> HHHHHHTPSTSVIPNDAIRLNQLGYYPNQEKIAVVDSGKVEEFVIWDAVSGEQVFVGKSLYTAKSAWSDKTRTTLDFSAVTTPGKYILKVNGASVTFLIKDSVLSPLA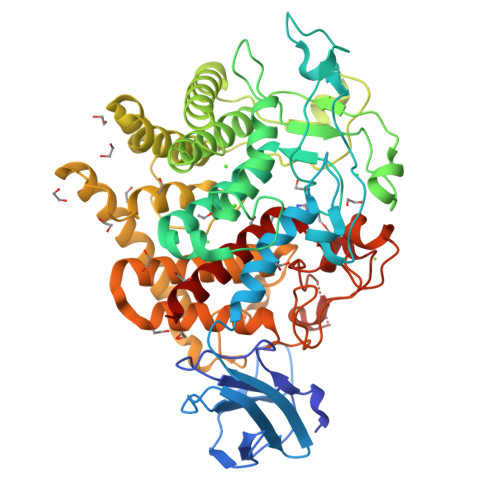DAALKSFYYQRTAMPIEEQYAGQWHRMAGHPDNHVLIHPSAASPDRPAGTIVSSSKGWYDAGDYNKYIVNSGYSIGLMQSIYQLFLDYFSRQKINIPESNNHTPDLLDEMQFNLDWMLTMQDPEDGGVYHKLTTPFFEGFVKPVDCKQQRYVVQKSVTAALDFAAVMAQSSRLFASYEEDYPGFSKRALLAAEKAYAWAEKHPEAYYNQNLLNQKYQPAIATGEYGDTHADDEFFWAASELYFSTGKEIYREEAIKKAPQIYTAPGWGNTFALGIFAWLQPGRELNEADRRFADSLKTELLKYADKVIEGAEQTPFHAPYGNDAKDFFWGCLAEKCMNQGVSLMYAYLQTGKDVYLTNAYRNMDYILGRNATGFCYVTGLGTKSPKHPHHRLSASDDIEDPIPGFLVGGPNPGQQDGAFYPTASPDESYVDTEDSYASNEVAINWNAALVALASSLDALAV1-(3-BROMOPHENYL)-7-CHLORO-6-METHOXY-3,4-DIHYDROISOQUINOLINE | C16 H13 Br Cl N O | 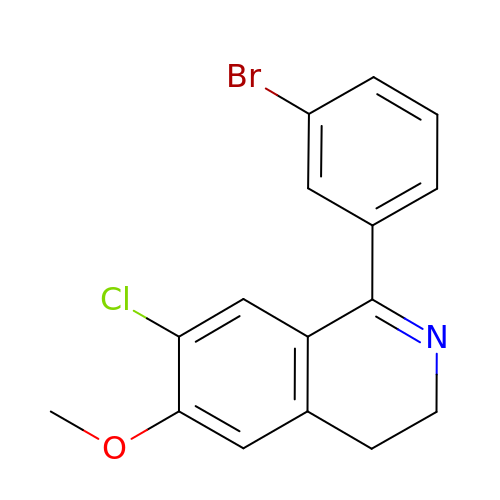IKGXHBGCVQTQBH-UHFFFAOYSA-N>[6x]X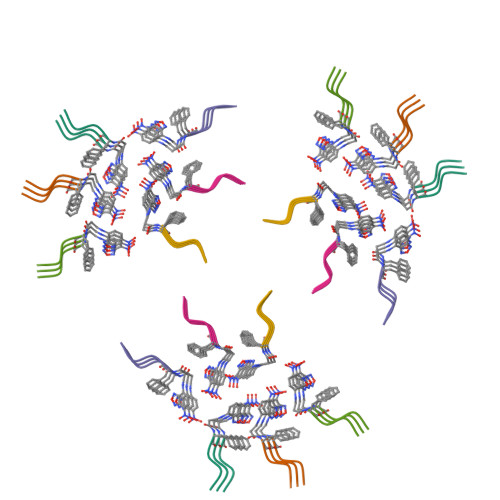FFSY> MKLKSFGVFGNPIKHSKSPLIHNACFLTFQKELRFLGHYHPILLPLESHIKSEFLHLGLSGANVTLPFKERAFQVCDKIKGIALECGAVNTLVLENDELVGYNTDALGFYLSLKQKNYQNALILGAGGSAKALACELKKQGLQVSVLNRSSRGLDFFQRLGCDCFMEPPKSAFDLIINATSASLHNELPLNKEVLKGYFKEGKLAYDLAYGFLTPFLSLAKELKTPFQDGKDMLIYQAALSFEKFSASQIPYSKAFEVMRSVFHHH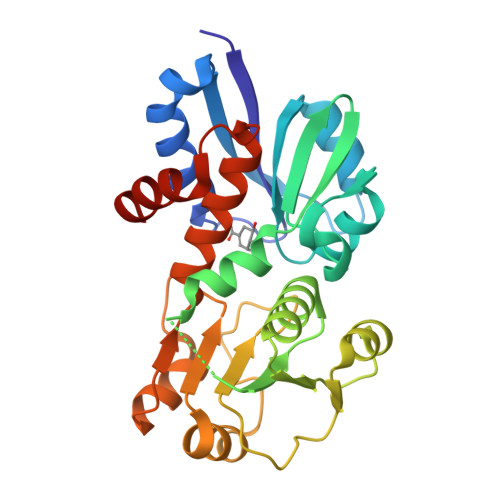HHH>[2x]SNSGSYNAR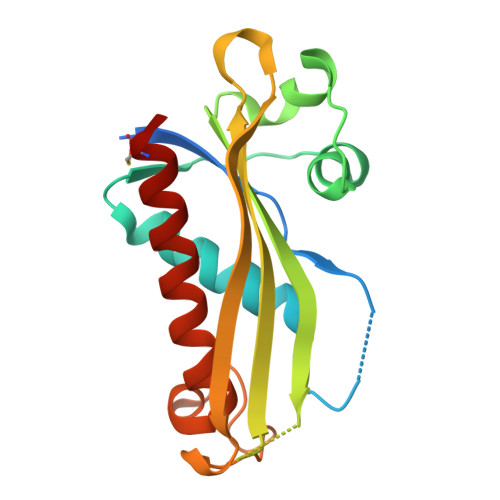LYTKGSKAKGVVAMLPVFYRTEKSAELLPWNLQAEFSEEISRRLHSSDKLLLIKHHASAGVAAQFFSPTPNISPELATQLLPAEFVVAAEILEQKTTEDVLNPSISASVRVRVFDIRHNKVSMIYQEILDASQSLASGSNDYHRYGWRSKNFDSTPMGLMHQRLFREIVARVEGYVCANYS>GSSHHHHHHSSGENLYFQGHMTCPFADPAALYSRQDTTSGQSPLAAYEVDDSTGYLTSDVGGPIQDQTSLKAGIRGPTLLEDFMFRQKIQHFD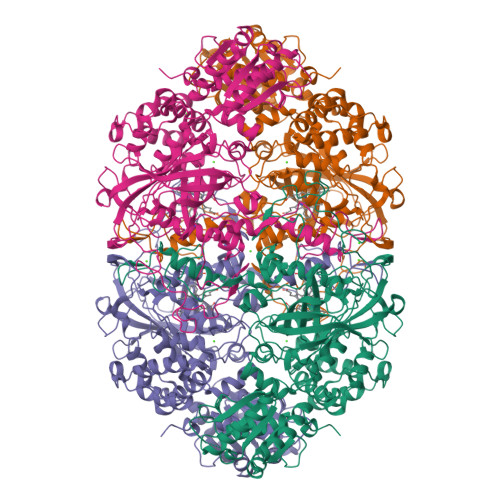HERVPERAVNARGAGAHGTFTSYADWSNITAASFLNATGKQTPVFVRFSTVAGSRGSADTARDVHGFATRFYTDEGNFDIVGNNIPVFFIQDAIQFPDLIHSVKPRPDNEIPQAATAHDSAWDFFSQQPSTMHTLFWAMSGHGIPRSYRHMDGFGVHTFRFVKDDGSSKLIKWHFKSRQGKASLVWEEAQVLSGKNADFHRQDLWDAIESGNGPEWDVCVQIVDESQAQAFGFDLLDPTKIIPEEYAPLTKLGLLKLDRNPTNYFAETEQVMFQPGHIVRGIDFTEDPLLQGRLFSYLDTQLNRNGGPNFEQLPINMPRVPIHNNNRDGAGQMFIHRNKYPYTPNTLNSGYPRQANQNAGRGFFTAPGRTASGALVREVSPTFNDHWSQPRLFFNSLTPVEQQFLVNAMRFEISLVKSEEVKKNVLTQLNRVSHDVAVRVAAAIGLGAPDADDTYYHNNKTAGVSIVGSGPLPTIKTLRVGILATTSESSALDQAAQLRTRLEKDGLVVTVVAETLREGVDQTYSTADATGFDGVVVVDGAAALFASTASSPLFPTGRPLQIFVDAYRWGKPVGVCGGKSSEVLDAADVPEDGDGVYSEESVDMFVEEFEKGLATFRFTDRFALDS[4x]> PMHPFVKALQEHFTAHQNPEKAEPMARYMKNHFLFLGIQTPERRQ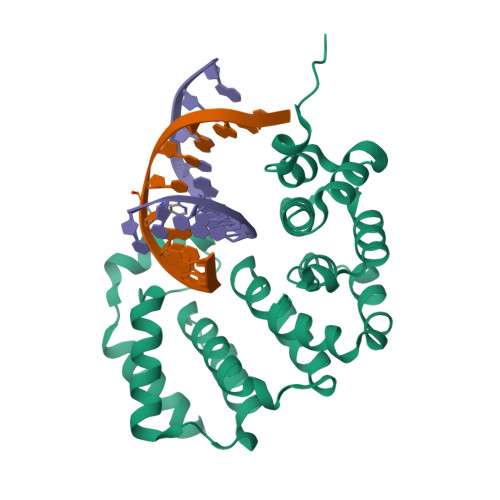LLKDIIQIHTLPDQKDFQIIIRELWDLPEREFQAAALDIMQKYKKHINETHIPFLEELIVTKSWWDSVDSIVPTFLGDIFLKHPELISAYIPKWIASDNIWLQRAAILFQLKYKQKMDEELLFWIIGQLHSSKEFFIQKAIGWVLREYAKTNPDVVWEYVQNNELAPLSKREAIKHIKQNYGINNEK(3S,4S,5R)-5-(hydroxymethyl)-3,4-bis(oxidanyl)piperidin-2-one | C6 H11 N O4 | 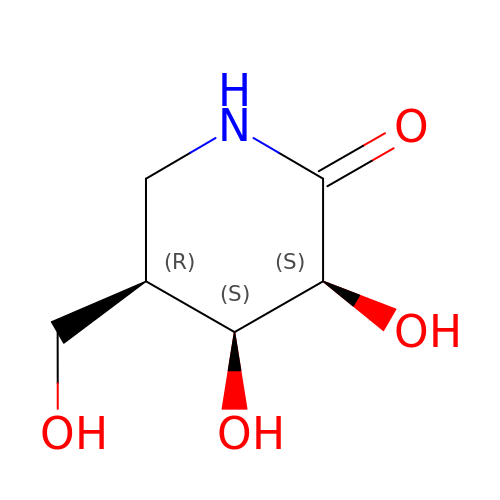ARBXEMIAJIJEQI-WISUUJSJSA-N>SSKEVAELKKQVESAELKNQRLKEVFQTKIQEFRKACYTLTGYQIDITTENQYRLTSLYAEHPGDCLIFKATSPSGSKMQLLETEFSHTVGELIEVHLRRQDSIPAFLSSLTLELFSRQTVA[4x];>KVQPSPTVHTKEALGFIMNMFQAPTS[4x]

The Mad1‐Mad2 complex, which is required to catalyse MCC formation, is targeted to kinetochores through a direct interaction with the phosphorylated conserved domain 1 (CD1) of Bub1. Mad1CTD is comprised of an N‐terminal elongated coiled‐coil, followed by a globular head domain featuring a conserved RWD (RING, WD40, DEAD) domain. Each monomer contains a long N‐terminal α‐helix (α1) forming the stem, followed by an antiparallel β‐sheet of four β‐strands (β1–4), a short helix (α2) and two C‐terminal helices (α3/α4). Bub1CD1 is largely a single α‐helix, consisting of almost four turns.

In each case, the asymmetry of the homodimer was retained. In the more asymmetric complex, there is a more marked difference in Bub1CD1 peptide occupancy, with high occupancy for the peptide bound to the concave side of the Mad1CTD coiled‐coil, and very low occupancy for the Bub1CD1 peptide bound to the convex side of the Mad1CTD coiled‐coil. Electron density map of the second homodimer from the Mad1CTD‐Bub1CD1 structure (shown directly above) from the P21 space group visualized in Coot. The occupancy of the peptide on the right is extremely poor as is the density for the head domain it contacts. Thus, this peptide is likely to bind with higher affinity and to represent the single binding peptide in solution as detected by NMR, ITC and AUC analyses. This model is supported by our Mad1CTD‐Bub1CD1 structures from various space groups where higher occupancy of the second Bub1CD1 peptide correlates with a more symmetric Mad1CTD dimer (Fig EV4).> PQFSLWKRPVVTAYIEGQPVEVLLDTGADDSIVAGIELGNNYSPKIVGGIGGFINTKEYKNVEIEVLNKKVRATIMTGDTPINIF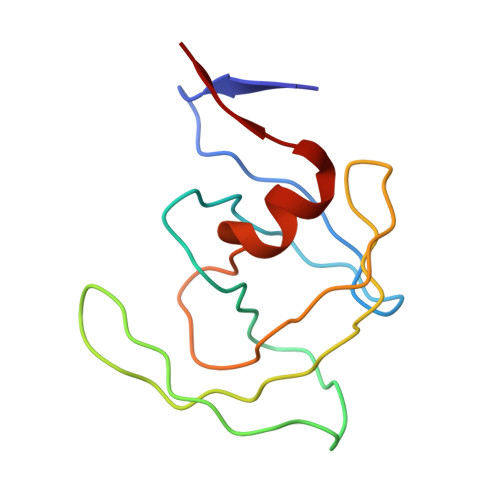GRNILTALGMSLNL>[2x]MPKVGIAAQAGRTRVRRAWLTALMMTAVMIGAVACGSGRGPAPIKVIADKGTPFADLLVPKLTASVTDGAVGVTVDAPVSVTAADGVLAAVTMVNDNGRPVAGRLSPDGLRWSTTEQLGYNRRYTLNATALGLGGAATRQLTFQTSSPAHLTMPYVMPGDGEVVGVGEPVAIRFDENIADRGAA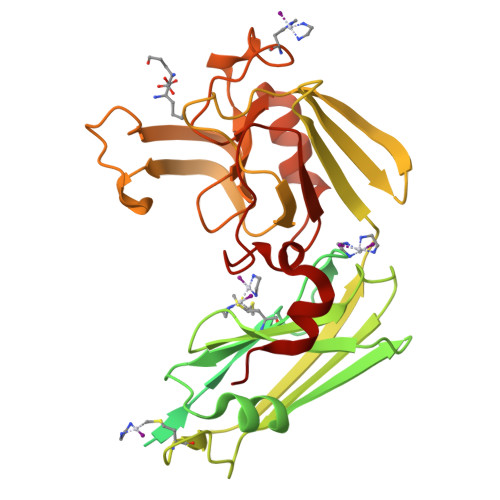EKAIKITTNPPVEGAFYWLNNREVRWRPEHFWKPGTAVDVAVNTYGVDLGEGMFGEDNVQTHFTIGDEVIATADDNTKILTVRVNGEVVKSMPTSMGKDSTPTANGIYIVGSRYKHIIMDSSTYGVPVNSPNGYRTDVDWATQISYSGVFVHSAPWSVGAQGHTNTSHGCLNVSPSNAQWFYDHVKRGDIVEVVNTVGGTLPGIDGLGDWNIPWDQWRAGNAKA>LEQKLISEEDLRSDKFRIMVQFLQANQESFMNGICGIMALASAQMYSSFEFTCPCLPDYNYAYGIGILIVPPIWFFLLGYVMNNNISVLTEEWKRPVGKRSKDPAVLRYMFSSMTQRALIAPAVWIAVTLMDGKSFLCAFSPTADLSEFVNESYQSLSQKELLKIQAKIPCKDIFEEHEIISREAATRYIRCLSQACGWTFLMVITLVAFLVRAIRPCFTQAAFLKTKYWSHYIDTERKLFDETCKEHAKSFAKVCIQQYFESISGEIVSQLPQSPAKKGKGNKDEDGEKQKSDEERLLGIRKEGDMNKVLWNWHTCKPPLLLSKRTEEMNGHAHLDTHSLTDERHTKKKAVVYYSKV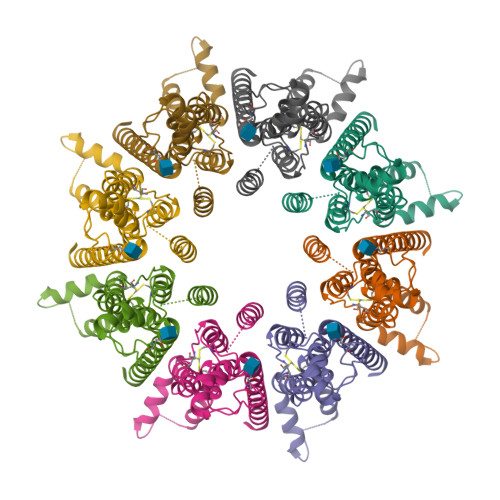[8x]> EFIEIVERSNYMGNPWTEYMAKYDIEEVHGSGIRVDLGEDAEVAGTQYRLPSGKCPVFGKGIIIENS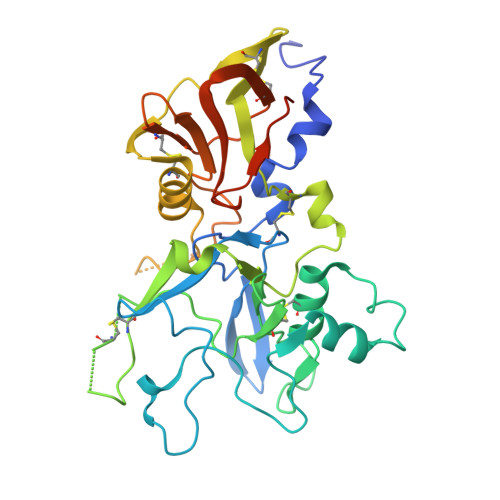KTTFLKPVATGNQDLKDGGFAFPPTNPLISPMTLNGMRDFYKNNEYVKNLDELTLCSRHAGNMNPDNDKNSNYKYPAVYDYNDKKCHILYIAAQENNGPRYCNKDQSKRNSMFCFRPAKDKLFENYVYLSKNVVDNWEEVCPRKNLENAKFGLWVDGNCEDIPHVNEFSANDLFECNKLVFELSASDQPKQYEQHLTDYEKIKEGFKNKNADMIKSAFLPTGAFKADRYKSHGKGYNWGNYNRETQKCEIFNVKPTCLINDKSYIATTALSHPIEVEHNFPGLEQKLISEEDLNSAVDHHHHHH> QPRRKLCILHRNPG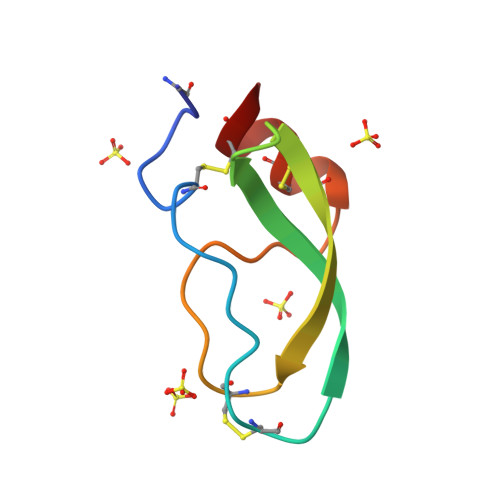RCYDKIPAFYYNQKKKQCERFDWSGCGGNSNRFKTIEECRRTCIG>[2x]GGSHMELPGSSMKPSGEDQAALAAGPWEECFQAAVQLALRAGQIIRKALTEEKRVSTKTS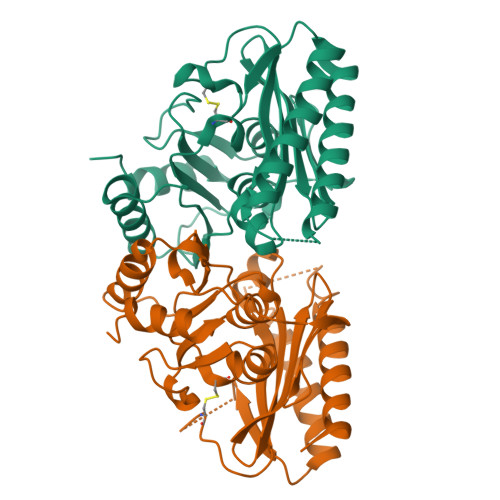AADLVTETDHLVEDLIISELRERFPSHRFIAEEAAASGAKCVLTHSPTWIIDPIDGTCNFVHRFPTVAVSIGFAVRQELEFGVIYHCTEERLYTGRRGRGAFCNGQRLRVSGETDLSKALVLTEIGPKRDPATLKLFLSNMERLLHAKAHGVRVIGSSTLALCHLASGAADAYYQFGLHCWDLAAATVIIREAGGIVIDTSGGPLDLMACRVVAASTREMAMLIAQALQTINYGRDDEK>[3x]MGHHHHHHHHMKFDNDSEKQVFDKLKKAIPGIIKEKCAGYDELYGYK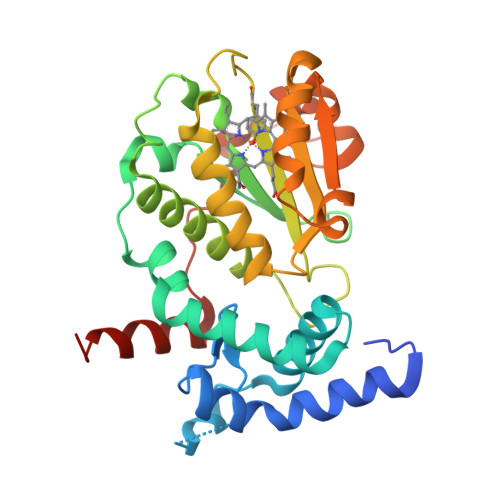LNPEGLTQEEVDKYYDEKIADRLTYKLCKAYQFEYSTIVQNLIDILNWRREFNPLSCAYKEVHNTELQNVGILTFDANGDANKKAVTWNLYGQLVKKKELFQNVDKFVRYRIGLMEKGLSLLDFTSSDNNYMTQVHDYKGVSVWRMDSDIKNCSKTVIGIFQKYYPELLYAKYFVNVPTVFGWVYDLIKKFVDETTRKKFVVLTDGSKLGQYLKDCPYEGYGGKDKKNNLTKQNVTNVHPTEYGLYILQKQIIEDVE(2R)-2-[5-CYCLOPROPYL-6-(HYDROXYSULFANYL)-4-(NAPHTHALEN-1-YLMETHYL)-2-OXOPYRIDIN-1(2H)-YL]-3-PHENYLPROPANOIC ACID | C28 H25 N O4 S | 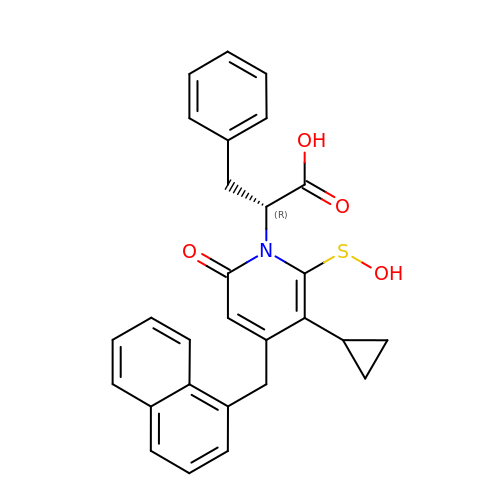RDAFPBNHIKAVPQ-DEOSSOPVSA-N>[3x]GAMQGEVSKAASADSTTEGTPADGFTVLSTKSLFLGQKLQVVQADIASIDSDAV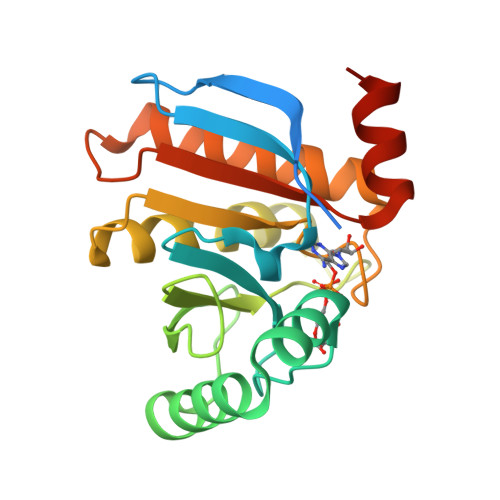VHPTNTDFYIGGEVGNTLEKKGGKEFVEAVLELRKKNGPLEVAGAAVSAGHGLPAKFVIHCNSPVWGADKCEELLEKTVKNCLALADDKKLKSIAFPSIGSGRNGFPKQTAAQLILKAISSYFVSTMSSSIKTVYFVLFDSESIGIYVQEMAKLDAN>SVDHGFLVTRHSQTIDDPQCPSGTKILYHGYSLLYVQGNERAHGQDLGTAGSCLRKFSTMPFLFCNINNVCNFASRNDYSYWLSTPEPMPMSMAPITGENIRPFISRCAVCEAPAMVMAVHSQTIQIPPCPSGWSSLWIGYSFVMHTSAGAEGSGQALASPGSCLEEFRSAPFIECHGRGTCNYYANAYSFWLATIERSEMFKKPTPSTLKAGELRTHVSRCQVCMRRT[6x]

Basement membranes are extracellular structures of epithelia and endothelia that have collagen IV scaffolds of triple α-chain helical protomers that associate end-to-end, forming networks. At the C-termini, interactions occur between the trimeric NC1 domains of two protomers, forming a hexamer of these domains reinforced by sulfilimine cross-links. Recent studies in one of our laboratories revealed that the NC1 domains function as recognition modules, directing the selection and assembly of α-chains into protomers and networks.

In vitro studies have shown that α1NC1 can assemble into homohexamers. We grew crystals of self-assembled recombinant α1NC1 subunits that diffracted X-rays to 1.8 Å resolution. Chloride ions were also present in our α1NC1homo, α3NC1homo and α5NC1homo structures at two different positions in the protomer–protomer interface. The very recent report of the existence of the α5NC1 homohexamer in vivo gives credence to the view that the canonical α1NC1 and α3NC1 homohexamers presented here may also exist in vivo, particularly given their structural stability, their proper binding of chloride ions for hexamer stabilization and their correct disposition of the residues that mediate the sulfilimine cross-linking bonds that stabilize the hexamer. The comparison of EA and EB of α3NC1 and α5NC1 also showed that they are identical in structure and also to the corresponding part of α1NC1, although no antigenicity has been determined in the latter chain in patients with Goodpasture’s disease.>[2x]MSYYHHHHHHLESTSLYKKAGLENLYFQGVKIMPNLPGLYFLQAYPSEEIWRLFVDGRFWSKENGWRGYESREPGCLNAALESLCSIALQVEKSGEEFELSVDLIKRIHKKCGKKVEELQEKNPGELRTDEPVSFGIPAGRASIKGIEEFLSLVFLTEGGAEFGPGKAGPFGPRFDKNYFKNLNPEQIPDLAKQIYFDMCKYGH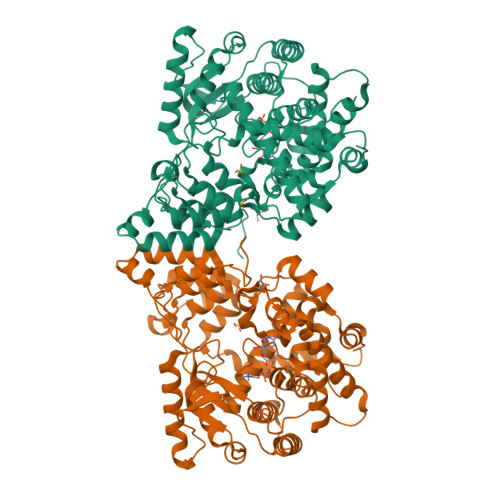SNTNHFYLAVMKNVDVYLEKITQSYNKEIKTAETLDEKLKIIVKHIRMYEVLAPFRDANGRTFVNNLLNIPLMQQGLPPATFYEPNVFDLYSAEELVVVVKEAIFNTVEIIEQSKRKTPITLYGYHSSLEEQTKFRDMLDSPSYEKIKHMDFSDLNPEKLHLKTQKCLSSLNEQYPLHRGAIYLSDPGEIKLLLSNRNESQINQQIEQGAPPIYVGKTPAHLAVISGNMAMLDELIAKKADLSLQDYDGKTALHYAAECGNMQIMGKILKVVLSQEDAIKVLNIKDNHGKTAFHYAAEFGTPELISAL> MAHSSATAGPQADYSGEIAELYDLVHQGKGKDYHREAADLAALVRRHSPKAASLLDVACGTGMHLRHLADSFGTVEGLELSADMLAIARRRNPDAVLHHGDMRDFSLGRRFSAVTCMFSSIGHLAG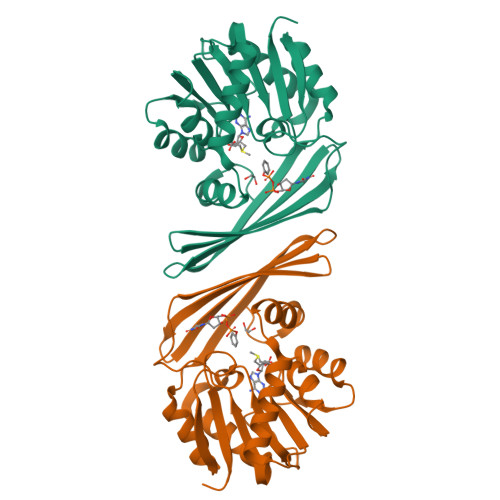QAELDAALERFAAHVLPDGVVVVEPWWFPENFTPGYVAAGTVEAGGTTVTRVSHSSREGEATRIEVHYLVAGPDRGITHHEESHRITLFTREQYERAFTAAGLSVEFMPGGPSGRGLFTGLPGAKGETRLEHHHHHH> MQFRSIIRIVGLLLALFSVTMLAPALVALLYRDGAGVPFVTTFFVLLFCGAMCWFPNRRHKHELKSRDGFLIVVLFWTVLGSAGSLPFLIADNPNISVTDAFFESFSALTTTGATVIVGLDELPKAILFYRQFLQWFGGMGIIVLAVAILPVLGIGGMQLYRAEIPGPVKDTKMTPRIAETAKALWYIYLSLTIACAVAFWLAGMTPFDAISHSFSTIAIGGFSTHDASMGYFDSYAINLITVVFLLISACNFTLHFAAFASGGVHPKYYWKDPEFRAFIFIQVLLFLVCFLLLLKHHSYTSPYDAFDQALFQTVSISTTAGFTTTGFADWPLFLPVLLLFSSFIGGCAGSTGGGMKVIRILLLTLQGARELKRLVHPRAVYTIKVGGSALPQRVVDAVWGFFS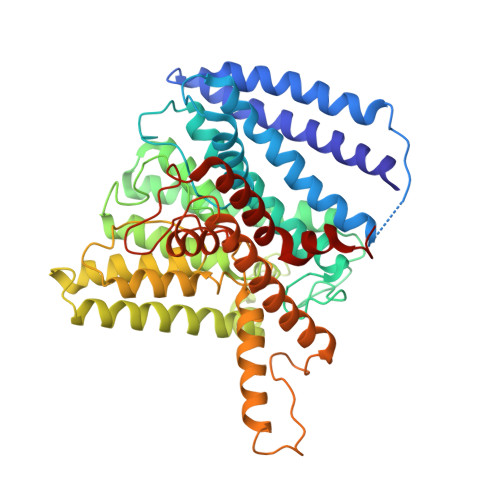AYALVFVVCMLGLIATGMDELSAFSAVAATLNNLGPGLGEVALHFGDVNDKAKWVLIVSMLFGRLEIFTLLILLTPTFWRS>[2x]MASSSTPRFRVYSKYLFLTYPQCTLEPQYALD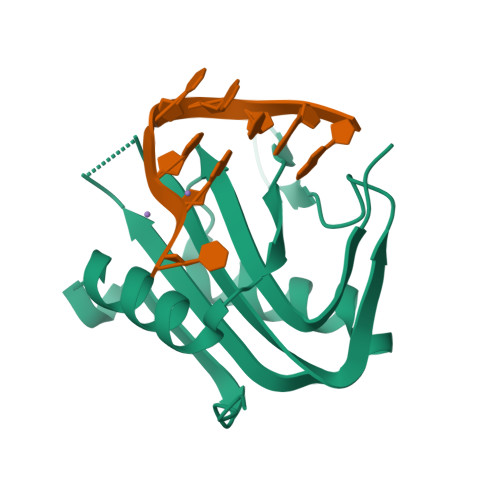SLRTLLNKYEPLYIAAVRELHEDGSPHLHVLVQNKLRASITNPNALNLRMDTSPFSIFHPNIQAAKDCNQVRDFITKEVDSDVNTAEWGTFVAVSTPGRKDRDADLE>[24x]MSELIVNVINGPNLGRLGRREPAVYGGTTHDELVALIEREAAELGLKAVVRQSDSEAQLLDWIHQAADAAEPVILNAGGLTHTSVALRDACAELS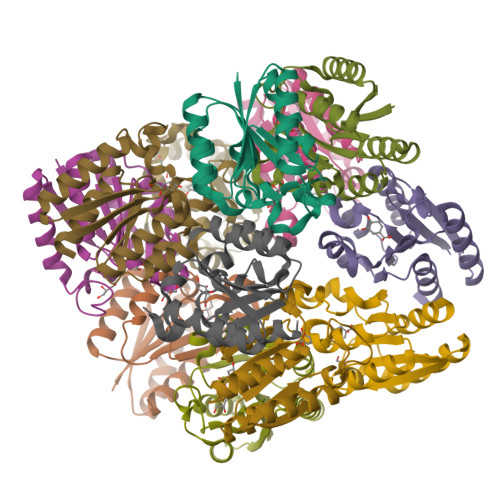APLIEVHISNVHAREEFRRHSYLSPIATGVIVGLGIQGYLLALRYLAEHVGT>LGKFSQTCYNSAIQGSVLTSTCERTNGGYNTSSIDLNSVIAAVDGSLKWQGSNFIEACRNTQLAGSSELAAECKTAAGQFVSTK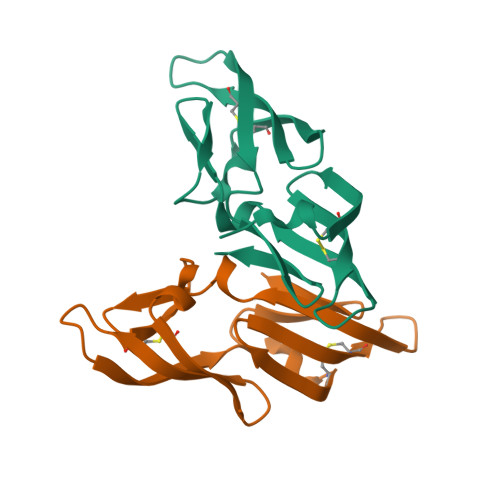INLDDHIANIDGTLKYE[2x]>[3x]SNAGGSSPITGLVYDQ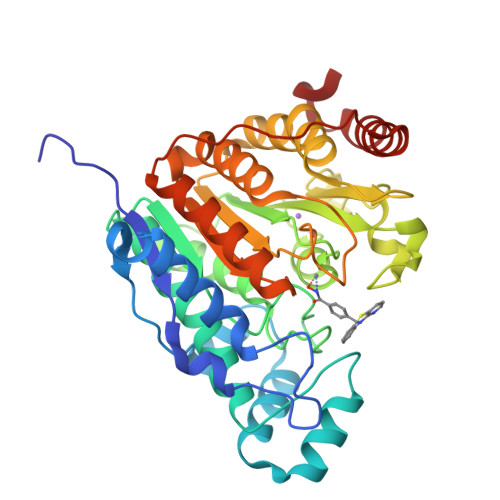RMMLHHNMWDSHHPELPQRISRIFSRHEELRLLSRCHRIPARLATEEELALCHSSKHISIIKSSEHMKPRDLNRLGDEYNSIFISNESYTCALLAAGSCFNSAQAILTGQVRNAVAIVRPPGHHAEKDTACGFCFFNTAALTARYAQSITRESLRVLIVDWDVHHGNGTQHIFEEDDSVLYISLHRYEDGAFFPNSEDANYDKVGLGKGRGYNVNIPWNGGKMGDPEYMAAFHHLVMPIAREFAPELVLVSAGFDAARGDPLGGFQVTPEGYAHLTHQLMSLAAGRVLIILEGGYNLTSISESMSMCTSMLLGDSPPSLDHLTPLKTSATVSINNVLRAHAPFWSSLR>[2x]HMLQPMAQALASLQGDDRVGVIEGRWIVFQPLAAPRSTGF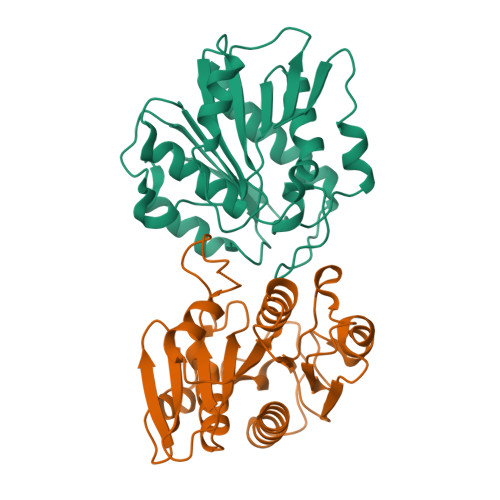IFYPGGRVDPRAYAPQARAIAEQGFLVVITPMPLNLAVFDADRASEVMAAFPEIEHWVIGGHSLGGAMAANFAHNHIGAVEGVVFWAAYPAQSDSLADRDDLTVYSIYGTLDGLATPDKIEASRALLPATARFIPIEGGNHAQFGWYGEQPGDNPATISRAQQQQMTVDATVEALAVVDGGFLEHHHHHH> ANLNGTLMQYFEWYMPNDGQHWKRLQNDSAYLAEHGITAVWIPPAYKGTSQADVGYGAYDLYDLGEFHQKGTVRTKYGTKGELQS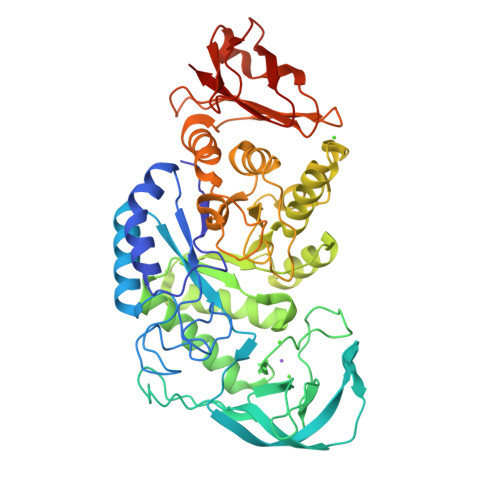AIKSLHSRDINVYGDVVINHKGGADATEDVTAVEVDPADRNRVISGEVLIKAWTHFHFPGRGSTYSDFKWHWYHFDGTDWDESRKLNRIYKFQGKAWDWEVSNEFGNYDYLMYADIDYDHPDVVAEIKRWGTWYANELQLDGFRLDAVKHIKFSFLRDWVNHVREKTGKEMFTVAEYWSYDLGALENYLNKTNFNHSVFDVPLHYQFHAASTQGGGYDMRKLLNGTVVSKHPLKSVTFVDNHDTQPGQSLESTVQTWFKPLAYAFILTRESGYPQVFYGDMYGTKGDSQREIPALKHKIEPILKARKQYAYGAQHDYFDHHDIVGWTREGDSSVANSGLAALITDGPGGAKRMYVGRQNAGETWHDITGNRSEPVVINSEGWGEFHVNGGSVSIYVQR The RecBCD complex of Escherichia coli plays a dual role in bacterial cell biology, acting both as a phage immunity hub and as the primary mechanism to initiate the recombinational repair of double-stranded DNA breaks (DSBs). The switch from the destructive to the recombinogenic mode is triggered during RecBCD translocation along DNA by recognition of a specific octameric ssDNA sequence called Chi (crossover hotspot instigator; 5′-GCTGGTGG-3′). Here, we present biochemical and structural analysis of two phage proteins, gp5.9 and Abc2, which target the DNA break resection complex RecBCD. These exemplify two contrasting mechanisms for control of DNA break repair in which the RecBCD complex is either inhibited or co-opted for the benefit of the invading phage.

We next solved cryoEM structures of the RecBCD-Abc2-PPI complex bound to a tailed DNA substrate. All of the particles within the dataset contained ordered density for RecBCD with additional density evident for the Abc2 protein. Focused classification with a mask around the phage binding site isolated 71% of the particles into a homogeneous class from which a 3.4 Å resolution structure of the RecBCD-Abc2-DNA complex was solved. From this class, a 3.8 Å resolution structure of RecBCD-Abc2-PPI-DNA complex was solved. The Abc2 protein adopts an extended alpha-helical structure and binds to the surface of the 'inactivated helicase domains' of RecC which play a key role in Chi recognition (Figure 4c–e, Figure 4—source data 1; Murphy, 2000). Consistent with biochemical observations, this location suggests a role for Abc2 in modulating the late stages of the DSB processing reaction catalysed by RecBCD (i.e. Chi recognition and associated conformational changes mediated by a 'latch' structure in RecC, or the subsequent loading of RecA protein). The binding site is also close to the interface with the helicase domains of RecB, and to a tunnel between RecB and RecC which has been suggested to allow exit of a recombinogenic ssDNA loop (the site of RecA loading) after Chi recognition. Additionally, Abc2 binding displaces a helical bundle, residues 252–294, from the RecC surface and some partial density can be seen for the displaced region clamping back over the exposed face of Abc2. Abc2 is bound to RecC in close proximity to both a 'latch helix' which is thought to control conformational changes in response to Chi, and to an 'alternative exit channel' in the RecBCD complex which is thought to accommodate a ssDNA loop in the post-Chi state (i.e. the recombinogenic mode). Given its location, it is plausible that Abc2 prevents RecA loading at this site and/or promotes the binding of Erf to the emerging ssDNA, but this remains to be tested experimentally.

> MPAPLYGADDPRRCSGNSVSEVLDKFRKNYDLIMSLPQETKEEKEFRHCIWLAEKEERERIYQTAIRPFRKATYTKFIEIDPRLRDYRSRYAGISNN;> MSDVAETLDPLRLPLQGERLIEASAGTGKTFTIAALYLRLLLGLGGSAAFPRPLTVEELLVVTFTEAATAELRGRIRSNIHELRIACLRETTDNPLYERLLEEIDDKAQAAQWLLLAERQMDEAAVFTIHGFCQRMLNLNAFESGMLFEQQLIEDESLLRYQACADFWRRHCYPLPREIAQVVFETWKGPQALLRDINRYLQGEAPVIKAPPPDDETLASRHAQIVARIDTVKQQWRDAVGELDALIESSGIDRRKFNRSNQAKWIDKISAWAEEETNSYQLPESLEKFSQRFLEDRTKAGGETPRHPLFEAIDQLLAEPLSIRDLVITRALAEIRETVAREKRRRGELGFDDMLSRLDSALRSESGEVLAAAIRTRFPVAMIDEFQDTDPQQYRIFRRIWHHQPETALLLIGDPKQAIYAFRGADIFTYMKARSEVHAHYTLDTNWRSAPGMVNSVNKLFSQTDDAFMFREIPFIPVKSAGKNQALRFVFKGETQPAMKMWLMEGESCGVGDYQSTMAQVCAAQIRDWLQAGQRGEALLMNGDDARPVRASDISVLVRSRQEAAQVRDALTLLEIPSVYLSNRDSVFETLEAQEMLWLLQAVMTPERENTLRSALATSMMGLNALDIETLNNDEHAWDVVVEEFDGYRQIWRKRGVMPMLRALMSARNIAENLLATAGGERRLTDILHISELLQEAGTQLESEHALVRWLSQHILEPDSNASSQQMRLESDKHLVQIVTIHKSKGLEYPLVWLPFITNFRVQEQAFYHDRHSFEAVLDLNAAPESVDLAEAERLAEDLRLLYVALTRSVWHCSLGVAPLVRRRGDKKGDTDVHQSALGRLLQKGEPQDAAGLRTCIEALCDDDIAWQTAQTGDNQPWQVNDVSTAELNAKTLQRLPGDNWRVTSYSGLQQRGHGIAQDLMPRLDVDAAGVASVVEEPTLTPHQFPRGASPGTFLHSLFEDLDFTQPVDPNWVREKLELGGFESQWEPVLTEWITAVLQAPLNETGVSLSQLSARNKQVEMEFYLPISEPLIASQLDTLIRQFDPLSAGCPPLEFMQVRGMLKGFIDLVFRHEGRYYLLAYKSNWLGEDSSAYTQQAMAAAMQAHRYDLQYQLYTLALHRYLRHRIADYDYEHHFGGVIYLFLRGVDKEHPQQGIYTTRPNAGLIALMDEMFAGMTLEEA;> MLRVYHSNRLDVLEALMEFIVERERLDDPFEPEMILVQSTGMAQWLQMTLSQKFGIAANIDFPLPASFIWDMFVRVLPEIPKESAFNKQSMSWKLMTLLPQLLEREDFTLLRHYLTDDSDKRKLFQLSSKAADLFDQYLVYRPDWLAQWETGHLVEGLGEAQAWQAPLWKALVEYTHQLGQPRWHRANLYQRFIETLESATTCPPGLPSRVFICGISALPPVYLQALQALGKHIEIHLLFTNPCRYYWGDIKDPAYLAKLLTRQRRHSFEDRELPLFRDSENAGQLFNSDGEQDVGNPLLASWGKLGRDYIYLLSDLESSQELDAFVDVTPDNLLHNIQSDILELENRAVAGVNIEEFSRSDNKRPLDPLDSSITFHVCHSPQREVEVLHDRLLAMLEEDPTLTPRDIIVMVADIDSYSPFIQAVFGSAPADRYLPYAISDRRARQSHPVLEAFISLLSLPDSRFVSEDVLALLDVPVLAARFDITEEGLRYLRQWVNESGIRWGIDDDNVRELELPATGQHTWRFGLTRMLLGYAMESAQGEWQSVLPYDESSGLIAELVGHLASLLMQLNIWRRGLAQERPLEEWLPVCRDMLNAFFLPDAETEAAMTLIEQQWQAIIAEGLGAQYGDAVPLSLLRDELAQRLDQERISQRFLAGPVNICTLMPMRSIPFKVVCLLGMNDGVYPRQLAPLGFDLMSQKPKRGDRSRRDDDRYLFLEALISAQQKLYISYIGRSIQDNSERFPSVLVQELIDYIGQSHYLPGDEALNCDESEARVKAHLTCLHTRMPFDPQNYQPGERQSYAREWLPAASQAGKAHSEFVQPLPFTLPETVPLETLQRFWAHPVRAFFQMRLQVNFRTEDSEIPDTEPFILEGLSRYQINQQLLNALVEQDDAERLFRRFRAAGDLPYGAFGEIFWETQCQEMQQLADRVIACRQPGQSMEIDLACNGVQITGWLPQVQPDGLLRWRPSLLSVAQGMQLWLEHLVYCASGGNGESRLFLRKDGEWRFPPLAAEQALHYLSQLIEGYREGMSAPLLVLPESGGAWLKTCYDAQNDAMLDDDSTLQKARTKFLQAYEGNMMVRGEGDDIWYQRLWRQLTPETMEAIVEQSQRFLLPLFRFNQS;> MKLQKQLLEAVEHKQLRPLDVQFALTVAGDEHPAVTLAAALLSHDAGEGHVCLPLSRLENNEASHPLLATCVSEIGELQNWEECLLASQAVSRGDEPTPMILCGDRLYLNRMWCNERTVARFFNEVNHAIEVDEALLAQTLDKLFPVSDEINWQKVAAAVALTRRISVISGGPGTGKTTTVAKLLAALIQMADGERCRIRLAAPTGKAAARLTESLGKALRQLPLTDEQKKRIPEDASTLHRLLGAQPGSQRLRHHAGNPLHLDVLVVDEASMIDLPMMSRLIDALPDHARVIFLGDRDQLASVEAGAVLGDICAYANAGFTAERARQLSRLTGTHVPAGTGTEAASLRDSLCLLQKSYRFGSDSGIGQLAAAINRGDKTAVKTVFQQDFTDIEKRLLQSGEDYIAMLEEALAGYGRYLDLLQARAEPDLIIQAFNEYQLLCALREGPFGVAGLNERIEQFMQQKRKIHRHPHSRWYEGRPVMIARNDSALGLFNGDIGIALDRGQGTRVWFAMPDGNIKSVQPSRLPEHETTWAMTVHKSQGSEFDHAALILPSQRTPVVTRELVYTAVTRARRRLSLYADERILSAAIATRTERRSGLAALFSSRE>[2x]MASSSTAYYLKDAGFHIRNIPKAWNDWNLFHVFQNFGKVSYCRVVGQSNDGQVQLGFVNMMSVADADEVRKNLNDGNLIGENFTLKVTDHKN;>[2x]DQENMLKISGYPGMLNTFGIAQLLTPYRVNGITITGAQSAVVALENKFQVYQAVQDFNGKKLDRNHKLQVSSLVVSSPAVPLE

By using functional proteomics, we and another group independently identified a piRNA biogenesis and chromosome segregation (PICS) complex (also named as PETISCO) that plays important roles in 21U-RNA biogenesis, chromosome segregation and cell division. The PICS complex is composed of TOFU-6, PICS-1 (also names as PID-3), ERH-2 and two mutually exclusive factors, PID-1 and TOST-1. The PID-1 containing complex is functional in piRNA maturation and processes piRNA precursors at 5′ termini via its association with IFE-3, while the TOST-1 containing form is essential for chromosome segregation and cell division in embryos. Complemented by biochemical and mutagenesis experiments, our structural biology data support that PICS is an octamer composed of two copies of each subunit, and unveil the assembly interface within PICS complex.

Consistent with previous work, PICS-1(PID-3) and TOFU-6 interact with each other via RRM domains, which were previously identified as the RNA binding modules. Given that the two structures are almost identical, the native one was used for structural analysis. TOFU-6C primarily interacts with PICS-1A through α1-β2 of TOFU-6C, and α2 and a C-terminal fragment of PICS-1A. α1 of TOFU-6C interacts with α2 of PICS-1A via both hydrophobic and electrostatic interactions. Specifically, Trp27, Phe30, His31, and Cys42 of TOFU-6C, make hydrophobic interactions with Lys246, Phe247, and Tyr250 of PICS-1A. Asp26 and Gln34 of TOFU-6C form salt bridges with Lys246 and Gln254 of PICS-1A, respectively. TOFU-6C also contacts with the other protomer of PICS-1(PID-3) (PICS-1B). The N-terminus and α2 of TOFU-6C interact with two loops of PICS-1B, one between β1 and α1 and the other between α2 and β4. Tyr8 and Leu10 of TOFU-6C make hydrophobic contacts with Pro211, Met213, and His265 of PICS-1B. Asp12 and Asp67 of TOFU-6C form salt bridges with Arg263 of PICS-1B. The PICS-1(PID-3) F217E mutant, which disrupts the homodimerization, failed to associate with perinuclear granules.> MSSTVISRKRRNSTVTEPDSSGETRKQKKSRSDEKSSSSKDGDPQLEFKVLQGYRDLESEMHKGRAQVTRTGDIGVAMDNLNAVDSLFNKVIGIKNNGLFAHDARAMVSISELAQISVRNLKFDDSRSMVNLENIVNSLKRYMLKEHFKLNNIAENRNDLTLAADEQSAADQQEESDGDIDRTPDDNHTDKATSSFKATSMRHSYLQQFSHYNEFSQFNWFRIGALYNTISKNAPITDHLMGPLSIEKKPRVLTQRRRNNDQVGEKITAEKITQHSLNSTQQETTPEQVKKCFKKLSKKLGPEGSINLFKFIIDPNSFSRSIENLFYTSFLIKEGKLLMEHDEEGLPTIKIKQSISHTDSRSKEIERQRRRAAHQNHIIFQMDMPTW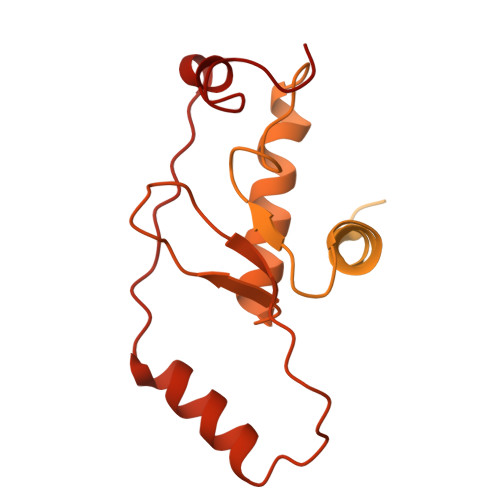RKLIKKYNITSPFLD>SMQKQAKEIKKHLFLLGGHDLEMQTIVQILTDRNVIFKDRYLQWDNALLSQYEEEIQQYGNKEPFIIYGVELKEDITPPTNYIRIDHHNEYATYPSALEQVASILDHPLNRYQTLVAANAKAYIPGMLEIGASHEEINLIRQEDRKAQGVIEDDEKLAQEAITNGT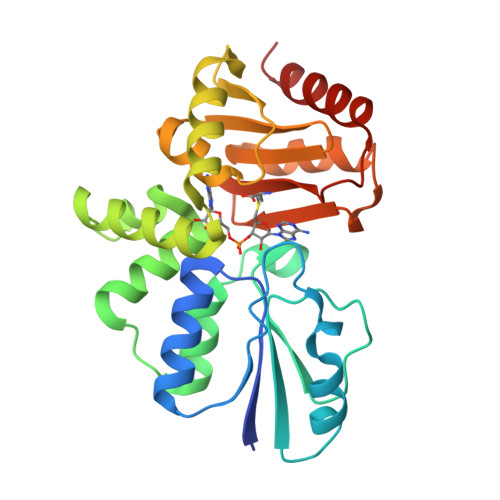EKIGSLYVVFTTANKFSPICDRLYPYEKLLIYTPNELIYYGKGINSIQKILKRYTPISNIFWGGGINGFIGTVRNRLTTNEILNIVEQIKLLEL[4x]> TGERGR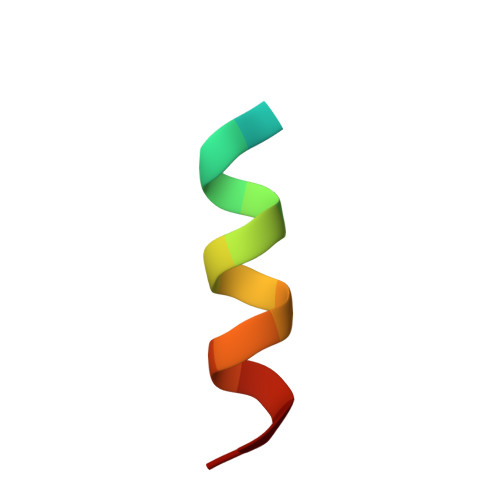WQVWGLAKRC>[4x]GPMEGECRVLSIQSHVVRGYVGNRAAMFPLQVLGFEVDAVNSVQFSNHTGYAHWKGQVLKSQELHELYEGLKVNDVNKYDYVLTGYTRDKSFLAMVVDIVRELKQQNSRLVYVCDPVMGDKWNGEGSMYVPQDLLPVYRDKVVPVADIITPNQFEAELLSGRKIHSQE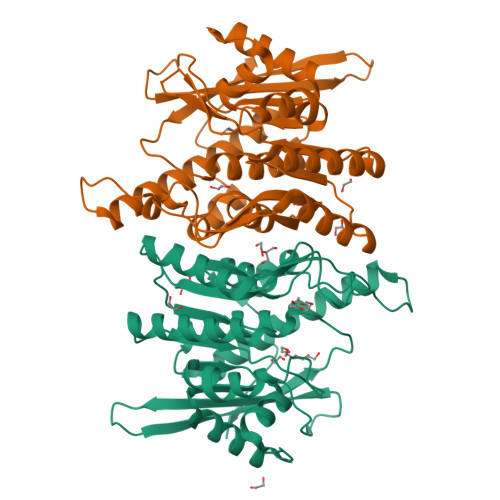EAFEVMDMLHCMGPDTVVITSSDLPSSQGSDYLIALGSQRMRKPDGSTVTQRIRMEMRKVEAVFVGTGDLFAAMLLAWTHKHPDNLKVACEKTVSAMQHVLQRTIRCAKAEAGEGQKPSPAQLELRMVQSKRDIEDPEIVVQATVL>MRGSHHHHHHGMASMRILLSNDDGVHAPGIQTLAKALREFADVQVVAPDRNRSGASNSLTLESSLRTFTFDNGDIAVQMGTPTDCVYLGVNALMRPRPDIVVSGINAGPNLGDDVIYSGTVAAAMAGRHLGFPALAVSLNGYQHYDTA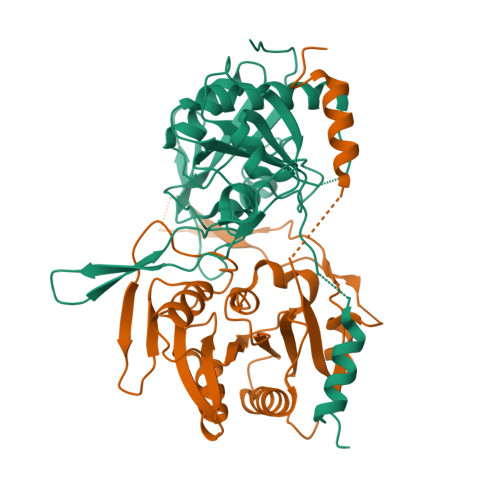AAVTCALLRGLSREPLRTGRILNVNVPDLPLAQVKGIRVTRCGSRHPADKVIPQEDPRGNTLYWIGPPGDKYDAGPDTDFAAVDEGYVSVTPLHVALTAHSAHDVVSDWLDSVGVGTQW[2x]>ADVEKHLELGKKLLAAGQLADALSQFHAAVDGDPDNYIAYYRRATVFLAMGKSKAALPDLTKVIALKMDFTAARLQRGHLLLKQGKLDEAEDDFKKVLKSNPSEQEEKEAESQLVKADEMQRLRSQALDAFDGADYTAAITFLDKILEVCVWDAELRELRAECFIKEGEPRKAISDLKAASKLKSDNTEAFYKISTLYYQLGDHELSLSEVRECLKLDQDHKRCFAHYKQVKKLNKLIESAEELIRDGRYTDATSKYESVMKTEPSVAEYTVRSKERICHCFSKDEKPVEAIRICSEVLQMEPDNVNAL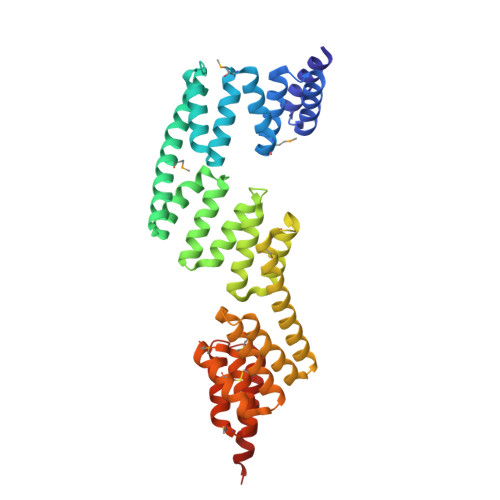KDRAEAYLIEEMYDEAIQDYEAAQEHNENDQQIREGLEKAQRLLKQSQKR[2x]>[48x]MTMQIKIKYLDET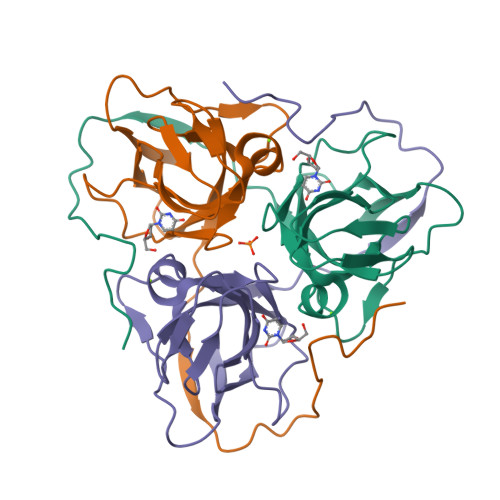QTRISKIEQGDWIDLRAAEDVTIKKDEFKLVPLGVAMELPEGYEAHVVPRSSTYKNFGVIQTNSMGVIDESYKGDNDFWFFPAYALRDTEIKKGDRICQFRIMKKMPAVELVEVEHLGNEDRGGLGSTGTK> MKFCIIGYPVRHSISPRLYNEYFKRAGMN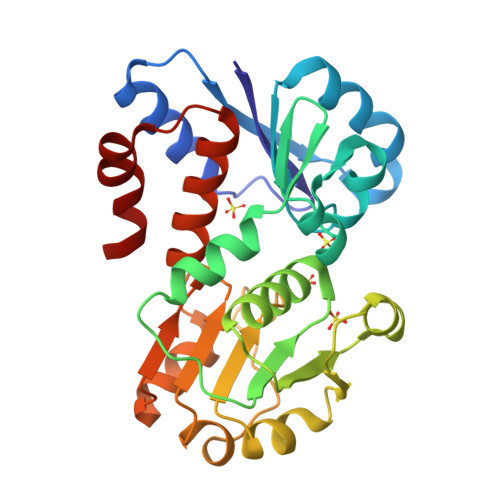HSYGMEEIPPESFDTEIRRILEEYDGFNATIPHKERVMRYVEPSEDAQRIKAVNCVFRGKGYNTDWVGVVKSLEGVEVKEPVVVVGAGGAARAVIYALLQMGVKDIWVVNRTIERAKALDFPVKIFSLDQLDEVVKKAKSLFNTTSVGMKGEELPVSDDSLKNLSLVYDVIYFDTPLVVKARKLGVKHIIKGNLMFYYQAMENLKIWGIYDEEVFKEVFGEVLK> MKFGIQFVPNEPIQKLCYYVKLAEDN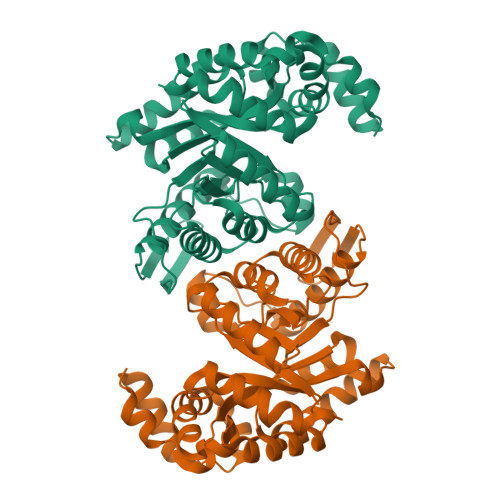GFEYCWITDHYNNRNVYMALTAIAMNTNKIKLGPGVTNPYVRSPAITASAIATLDELSGGRAVLGIGPGDKATFDALGIEWVKPVTTLKESIEVIRKLLAGERVSYEGKVVKIAGAALAVKPIQKAVPVYMGAQGPKMLETAGMIADGVLINASNPKDFEAAIPLIKKGAEAAGRSMDEIDVAAYACMSVDKNADKAKQAAVPVVAFIAAGSPPVVLERHGIDMEKVEAIRNALKSGNFPEAFKNVDDTMLEAFSIYGTPEDVVEKCKKLAEMGVTQIVAGSPIGPNKETAIKLIGKKVIPALKE The photoreceptor sensory rhodopsin II from N. pharaonis (NpSRII) in complex with its cognate transducer NpHtrII serves as a model system for studying transmembrane signal transfer. This complex displays a 2:2 stoichiometry where two transducers are flanked by two receptors. The long rod-shaped cytoplasmic domain consists of two HAMP domains (present in Histidine kinases, Adenyl cyclases, Methyl-accepting proteins and Phosphatases23), which are followed by a methylation domain4 involved in the adaptation processes and a signaling domain which harbors the CheW/CheA binding site5. HAMP subunits contain two amphiphilic helices (AS1 and AS2) joined by a non-helical connector.

Here, we report on new crystal structures of the ground and active M-state of NpSRII/NpHtrII1–157 complexes, in the space group I212121. Interestingly, the orientation of symmetrical parts of the dimer of two proteins is “U”-shaped contrary to the “V”-shaped quaternary structure reported previously (space group P21212). Having established that the fine structure of the proteins itself in the complex in the two crystal forms is unperturbed, we analyzed the overall structures in the crystal lattices. It is evident from Fig. 4 that the two receptors are oriented nearly parallel to the transducer and form a “U”-shaped binding crevice in the new crystal form I212121 compared to the “V”-shaped structure in the original P21212 symmetry. The angle between the G helices of NpSRII in the “U”-shape and the “V”-shape is 11°. A single NpSRII monomer of the “U”-shape dimer can be superimposed with the corresponding monomer of the “V”-shape dimer by a rigid body rotation by an angle of 8.5°. When comparing wild type structures solved in the I212121 and previously solved in the P21212 space groups it is seen that the structure of NpSRII is nearly the same (with backbone RMS deviation of 0.22 Å for ordered regions) and is highly similar to the structure of NpSRII when crystallized alone (with backbone RMS deviation of 0.27 Å for ordered regions). Having two data sets from different space groups (I212121 and P21212), we checked whether different crystal contacts have a structural influence on the retinal-binding site. As can be seen from Fig. 2 there are almost no differences found for the ground state structures as well as for the activated M intermediate, indicating that the different crystallization conditions and space groups have little, if any at all, influence on the functionally important regions within NpSRII. We found that only the “U”-shape structure allows a close interaction between NpSRII and the HAMP domain, allowing it to be compactly fitted into the “U”-shape topology. Here, we have presented the structure in the space group I212121, where the whole complex is more compact (quaternary structure has a “U”-shape) and the receptor can extensively interact with the transducer’s HAMP domain.

> VGLTTLFWLGAIGMLVGTLAFAWAGRDAGSGERRYYVTLVGISGIAAVAYVVMALGVGWVPVAERTVFAPRYIDWILTTPLIVYFLGLLAGLDSREFGIVITLNTVVMLAGFAGAMVPGIERYALFGMGAVAFLGLVYYLVGPMTESASQRSSGIKSLYVRLRNLTVILWAIYPFIWLLGPPGVALLTPTVDVALIVYLDLVTKVGFGFIALDAAATLRAEHGESLAGVDTDAPAVADENSHHHHHHH;> AVSRLLLPSRVRHSYTGKMGAVFIFVGALTVLFGAIAYGEVTAAAATGDAAAVQEAAVSAILGLIILLGINLGLVAATLGGDTAASLSTLAAKASRMGDGDLDVELETRREDEIGDLYAAFDEMRQSVRTSLEDAKNAREDAEQAQKRAEEINTNSHHHHHHH>[2x]CGCGAATTXG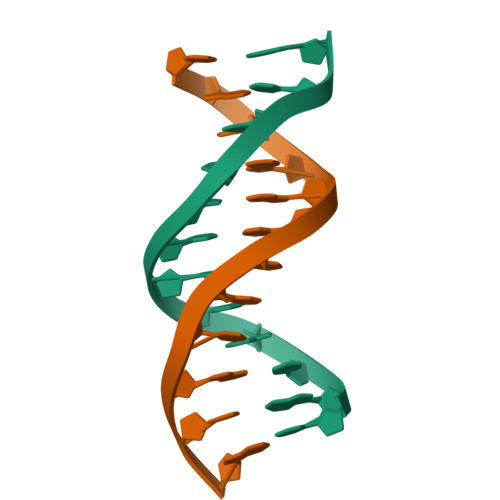CG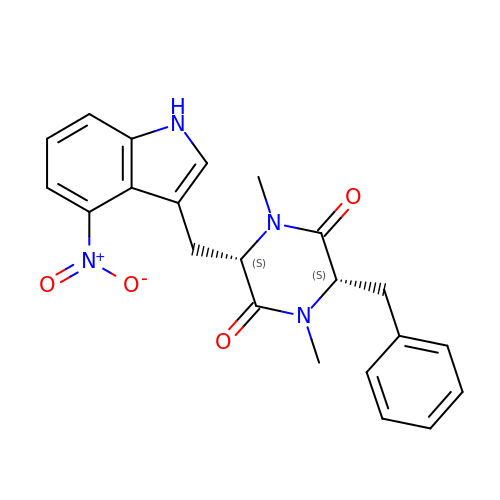(3~{S},6~{S})-1,4-dimethyl-3-[(4-nitro-1~{H}-indol-3-yl)methyl]-6-(phenylmethyl)piperazine-2,5-dione | C22 H22 N4 O4 | GJJXGBLNXDIHIQ-OALUTQOASA-N> GPSRGAQNSISWEVQRFDGWYNNLMEHRWGSKGSRLQRLVPASYADGVYQPLKEPYLPNPRHLSNRVMRGSAGQPSLRNRTVLGVFFGYHVLSDLVSVETPGCPAEFLNIYIPHGDPVFDPDKRGNVVLPFQRSRWDRNTGQSPSNPRDQSNQVTGWLDGSAIYGSSHSWSDTLRSFSGGQLASGPDPAFPSDSQSSLLMWMAPDPSTGQGGPRGVYAFGAQRGNREPFLQALGLLWFRYHNLCARKLAQEHPHWGDEELFQHARKRVIATYQNIAMYEWLPSFLKQTPPEYPGYRPFLDPSISPEFVVASEQFLSTMVPSGVYMRNASCHFQGIPSHNSSVSGALRVCNSYWSREHPKLQRAEDVDALLLGMASQIAEREDHVVVEDMQDFWPGPLKFSRTDYLASCLQRGRDLGLPSYTKAREALGLSPISHWQDINPALSRSNGTVLEATAALYNQDLSRLELLPGGLLESHGDPGPLFSTIVLDQFVRLRDGDRYWFENTRNGLFSKEEIAEIRNTSLRDILVAVTNVDPSALQPNVFFWLAGDPCPQPSQLSAKGLPACAPLFIRDYFEGSGFGFGLTIGTLCCFPLVSLLSAWIVARLRKRNFKRLQRQDRQSIMSEKLVGGVEALEWQGRNEPCRPVLVHLQPGQIRVVDGRLTVLRTIQLRPPQQVNLILSSNRGRRTLLLKIPKEYDLVLLFNMEEERQALVENVRGALKENGLSFQEWELREQELMRAAVTRQQRGHLLETFFRHLFSQVLDINQADAGTLPLDSSTKVREALTCELSRAEFADSLGLKPQDMFVESMFSLADKDGNGYLSFREFLDILVVFMKGSPEEKSRLMFRMYDFDGNGLISKDEFIRMLRSFIEISNNCLSKAQLAEVVESMFRESGFQDKEELTWEDFHFMLRDHDSDLRFTQLCVKGVEVPEVIKNLCRRASYISQEKICPSPRMSAHCARNNMKTASSPQRLQCPMDTDPPQEIRRRFGKKVTSFQPLLFTEAHREKFQRSRRHQTVQQFKRFIENYRRHIGCVAVFYTITGALFLERAYYYAFAAHHSGITDTTRVGIILSRGTAASISFMFSYILLTMCRNLITFLRETFLNRYIPFDAAVDFHRLIASTAIILTVLHSAGHVVNVYLFSISPLSVLSCLFPGLFHDDGSEFPQKYYWWFFQTVPGLTGVLLLLALAIMYVFASHHFRRRSFRGFWLTHHLYIFLYILLIIHGSFALIQMPRFHIFFLVPAIIYVGDKLVSLSRKKVEISVVKAELLPSGVTHLRFQRPQGFEYKSGQWVRIACLALGTTEYHPFTLTSAPHEDTLSLHIRAAGPWTTRLREIYSPPTGDTCARYPKLYLDGPFGEGHQEWHKFEVSVLVGGGIGVTPFASILKDLVFKSSVSCQVFCKKIYFIWVTRTQRQFEWLADIIREVEENDRQDLVSVHIYITQLAEKFDLRTTMLYICERHFQKVLNRSLFTGLRSITHFGRPPFEPFFNSLQEVHPQVRKIGVFSCGPPGMTKNVEKACQLINRQDRTHFSHHYENF;> MAALGHTLPFYTGTKPTFPMDTTLAVIITIFLTALVTFIIILPGIRGKTRLFWLLRVVTSLFIGAVILAVNFSSEWSVGHVNANTTYKAFSPKWVSVDVGL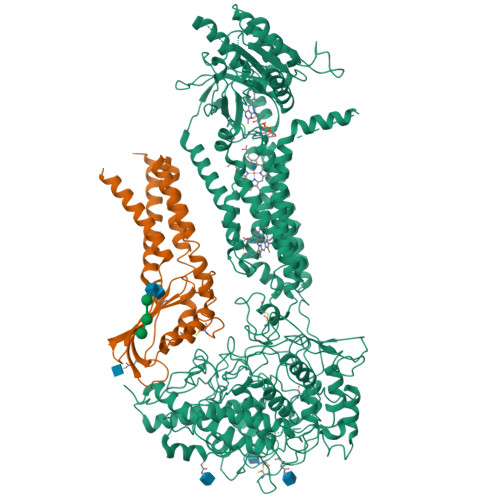QIGLGGVNITLTGTPVQQLNETINYNEAFAWRLGRSYAEEYAKALEKGLPDPVLYLAEKFTPRSPCGLYNQYRLAGHYASAMLWVAFLCWLLANVMLSMPVLVYGGHMLLATGLFQLLALFFFSMTTSLISPCPLRLGTAVLHTHHGPAFWITLATGLLCILLGLVMAVAHRMQPHRLKAFFNQSSEDPVLEWGSEEGGLLSPHYRSIAESPETQDIPMSVASSETCFKEEHPKESDCSL>[3x]MDHAPERFDATPPAGEPDRPALGVLELTSI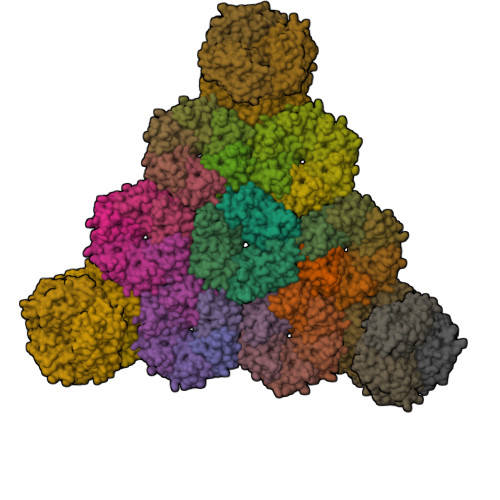ARGITVADAALKRAPSLLLMSRPVSSGKHLLMMRGQVAEVEESMIAAREIAGAGSGALLDELELPYAHEQLWRFLDAPVVADAWEEDTESVIIVETATVCAAIDSADAALKTAPVVLRDMRLAIGIAGKAFFTLTGELADVEAAAEVVRERCGARLLELACIARPVDELRGRLFF;>[18x]MSITLRTYIFLDALQPQLATFIGKTARGFLPVPGQASLWVEIAPGIAINRVTDAALKATKVQPAVQVVERAYGLLEVHHFDQGEVLAAGSTILDKLEVREEGRLKPQVMTHQIIRAVEAYQTQIINRNSQGMMILPGESLFILETQPAGYAVLAANEAEKAANVHLVNVTPYGAFGRLYLAGSEAEIDAAAEAAEAAIRSVSGVAQESFRDR;>[36x]MADALGMIEVRGFVGMVEAADAMVKAAKVELIGYEKTGGGYVTAVVRGDVAAVKAATEAGQRAAERVGEVVAVHVIPRPHVNVDAALPLGRTPGMDKSA>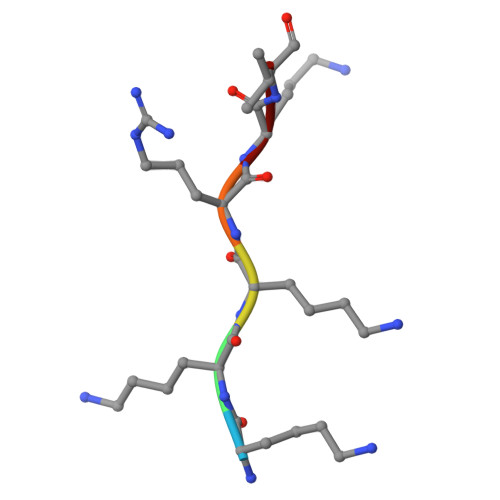 KKKRKV> TSDSTAPSALIDGPQTGFTMTNDGARTEPDEQDAVYDIMRATGNDWAAAIPDVCRGRWHGIE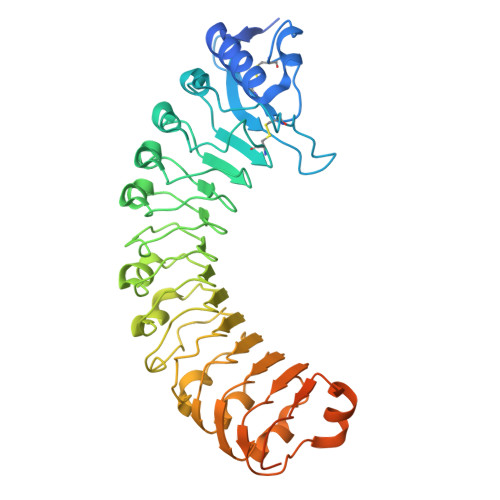CMPDQDNVYHVVSLSFGALSDDTAFPTCDPQRSYVSESLTRLKHLKALFFYRCLGRAPQRIPAFLGRLGSSLQTLVLRENGFLGPIPDELGNLTNLKVLDLHKNHLNGSIPLSFNRFSGLRSLDLSGNRLTGSIPGFVLPALSVLDLNQNLLTGPVPPTLTSCGSLIKIDLSRNRVTGPIPESINRLNQLVLLDLSYNRLSGPFPSSLQGLNSLQALMLKGNTKFSTTIPENAFKGLKNLMILVLSNTNIQGSIPKSLTRLNSLRVLHLEGNNLTGEIPLEFRDVKHLSELRLNDNSLTGPVPFERDTVWRMRRKLRLYNNAGLCVNRDSDLDDAFGSKSGSTVRLCDAETSRPAPSGTVQHLSREEDGAL>[2x]MRCTRAIRQTARTGWLTWLAILAVTAPVTSPAWADDPPATVYKYDSRPPEDVFQNGFTAWGNNDNVLEHLTGRSCQVGSSNSAFVSTSSSRRYTEVYLEHRMQEAVEAERAGRGTGHFIGYIYEVRADNNFYGAASSYFEYVDTYGDNAGRILAGALATYQSGYLAHRRIPPENIRRVTRVYHNGITGETTTTEYSNARYVSQQTRANPNPYTSRRSVASIVGTLVRMAPVVGACMARQAESSEAMAAWSERAGEAMVLVYYESIAYSF;>MPIDRKTLCHLLSVLPLALLGSHVARASTPGIVIPPQEQITQHGSPYGRCANKTRALTVAELRGSGDLQEYLRHVTRGWSIFALYDGTYLGGEYGGVIKDGTPGGAFDLKTTFCIMTTRNTGQPATDHYYSNVTATRLLSSTNSRLCAVFVRSGQPVIGACTSPYDGKYWSMYSRLRKMLYLIYVAGISVRVHVSKEEQYYDYEDATFETYALTGISICNPGSSLC[2x];>[2x]MLINNKKLLHHILPILVLALLGMRTAQAVAPGIVIPPK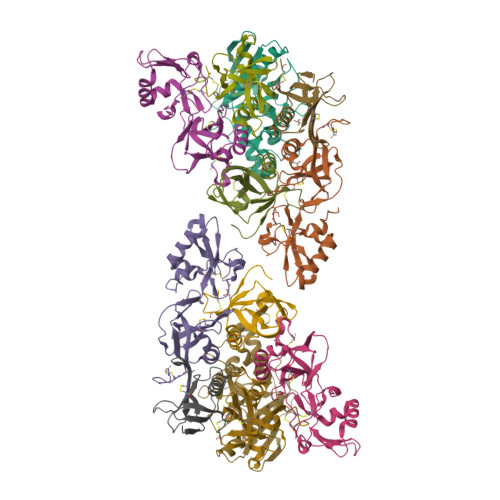ALFTQQGGAYGRCPNGTRALTVAELRGNAELQTYLRQITPGWSIYGLYDGTYLGQAYGGIIKDAPPGAGFIYRETFCITTIYKTGQPAADHYYSKVTATRLLASTNSRLCAVFVRDGQSVIGACASPYEGRYRDMYDALRRLLYMIYMSGLAVRVHVSKEEQYYDYEDATFQTYALTGISLCNPAASIC;>MLRRFPTRTTAPGQGGARRSRVRALAWLLASGAMTHLSPALADVPYVLVKTNMVVTSVAMKPYEVTPTRMLVCGIAAKLGAAASSPDAHVPFCFGKDLKRPGSSPMEVMLRAVFMQQRPLRMFLGPKQLTFEGKPALELIRMVECSGKQDCP[4x];>MQRQAGLPLKANPMHTIASILLSVLGIYSPADVAGLPTHLYKNFTVQELALKLKGKNQEFCLTAFMSGRSLVRACLSDAGHEHDTWFDTMLGFAISAYALKSRIALTVEDSPYPGTPGDLLELQICPLNGYCE[2x]>[2x]MSLGHIIVTGAGSGLGRALTIGLVERGHQVSMMGRRYQRLQQQELLLGNAVIGIVADLAHHEDVDVAFA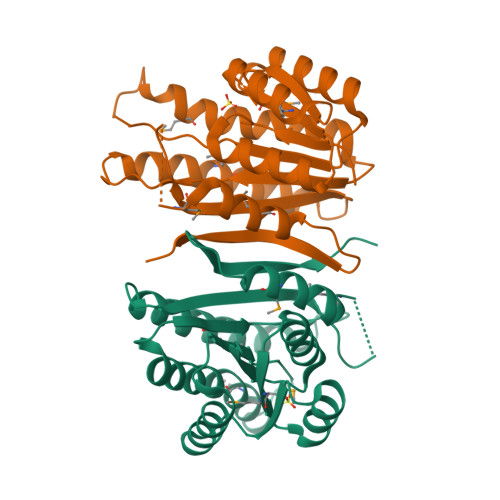AAVEWGGLPELVLHCAGTGEFGPVGVYTAEQIRRVMESNLVSTILVAQQTVRLIGERGGVLANVLSSAAQVGKANESLYCASKWGMRGFLESLRAELKDSPLRLVNLYPSGIRSEFWDNTDHVDPSGFMTPEDAAAYMLDALEARSSCHVTDLFIGRNEGHHHHHH> SSGLNDIFEAQKIEWHEGSAGGSGGSGRSSLDNIEMAYARQIYIYNEKIVNGHLQPNLVDLCASVAELDDKSISDMWTMVKQMTDVLLTPATDALKNRSSVEVRMEFVRQALAYLEQSYKNYTLVTVFGNLHQAQLGGVPGTYQLVRSFLNIKLPAPLPGLQDGEVEGHPVWALIYYCMRCGDLLAASQVVNRAQHQLGEFKTWFQEYMNSKDRRLSPATENKLRLHYRRALRNNTDPYKRAVYCIIGRCDVTDNQSEVADKTEDYLWLKLNQVCFDDDGTSSPQDRLTLSQFQKQLLEDYGESHFTVNQQPFLYFQVLFLTAQFEAAVAFLFRMERLRCHAVHVALVLFELKLLLKSSGQSAQLLSHEPGDPPCLRRLNFVRLLMLYTRKFESTDPREALQYFYFLRDEKDSQGENMFLRCVSELVIESREFDMILGKLENDGSRKPGVIDKFTSDTKPIINKVASVAENKGLFEEAAKLYDLAKNADKVLELMNKLLSPVVPQISAPQSNKERLKNMALSIAERYRAQGISANKFVDSTFYLLLDLITFFDEYHSGHIDRAFDIIERLKLVPLN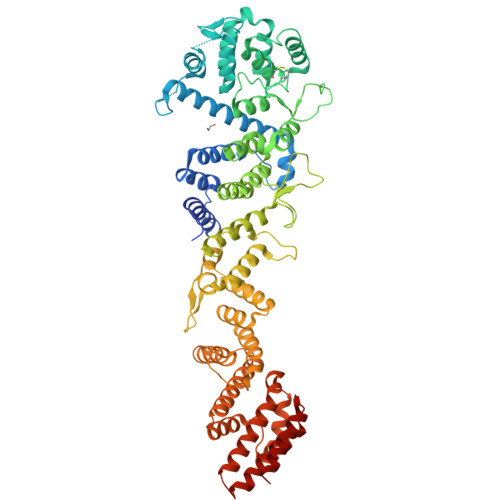QESVEERVAAFRNFSDEIRHNLSEVLLATMNILFTQFKRLKGTSPSSSSRPQRVIEDRDSQLRSQARTLITFAGMIPYRTSGDTNARLVQMEVLMN>[2x]SLRSDLINALYDENQKYDVCGIISAEGKIYPLGSDTAVLSTIFELFSRPIINKIAEKHGYIVEEPKQQNHYPDFTLYKPSEPNKKIAIDIKTTYTNKENEK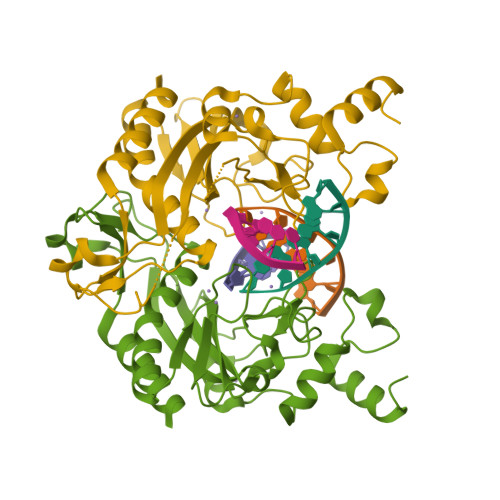IKFTLGGYTSFIRNNTKNIVYPFDQYIAHWIIGYVYTRVATRKSSLKTYNINELNEIPKPYKGVKVFLQDKWVIAGDLAGSGNTTNIGSIHAHYKDFVEGKGIFDSEDEFLDYWRNYERTSQLRNDKYNNISEYRNWIYRGRK> GPMSVPTDGAVTTSQIPASEQETLVRPKPLLLKLLKSVGAQKDTYTMKEVLFYLGQYIMTKRLYDEKQQHIVYCSNDLLGDLFGVPSFSVKEHRKIYTMIYRNLVVVNQQES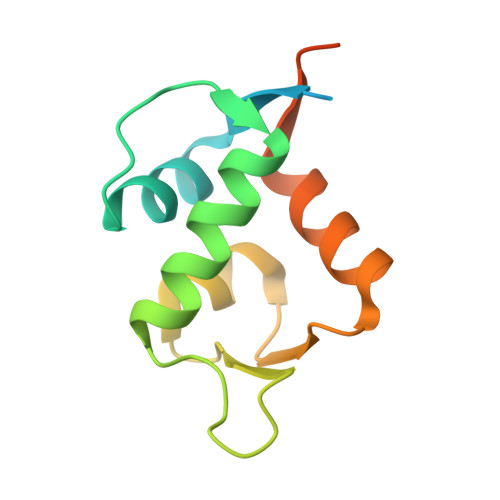SDSGTSVSEN> GEGKEDAF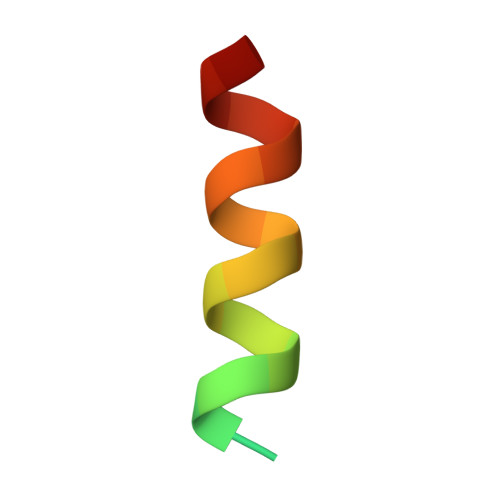SKLKEKFMNELHK>[18x]GAMGNQKTKASKLETAAKNLENQNKQEYIKINEIDAQGINFLATFKADEKDNLSQYEEMQIKRTIYSSLNYEKQKINTLKEILETLYNKLQHRYTSKEFIYQIVASIQYDIDRVLCLIKEAIIKDNLHTQNQKESELLMNLDSSLKTRQNFAKKLNETIDDYNKDSKNIQTNVDALATYMKENYKTLDSFKPIN

Two CspA orthologous proteins, BGA71 and BGA66, that are capable of binding complement system components C7, C8, and C9 and thus inhibiting the assembly of the MAC have been identified in B. bavariensis, allowing B. bavariensis to escape the attack by the immune system. The importance of BGA71 and BGA66 in the resistance to the immune system was supported by the gain of resistance to complement-mediated killing after expression of either protein in the serum-sensitive B. garinii strain G132. In conclusion, we have solved the crystal structure of the key complement inhibitory protein BGA71 from B. bavariensis. The overall fold of the BGA71 protein looks similar (Cα root-mean-square deviation from 1.66 Ǻ to 2.63 Ǻ) to the previously released crystal structures of the orthologous PFam54 proteins CspA, BBA64, BBA66, and BBA73 of B. burgdorferi.

All three BGA71 constructs were overexpressed in E. coli, but only BGA7162-251 yielded crystals, suggesting that the flexible region present in the other two constructs interfered with the crystal formation, as previously observed for the BBA66 protein of B. burgdorferi. The diffracting crystals of the Se-Met BGA7162-251 construct belonged to the space group P31 and contained 18 molecules per asymmetric unit with a water content of approximately 45%. The final model of BGA7162-251 was generated for residues 69–251 since the first four residues that remained after cleavage of the His-tag and residues 66–68 were not built due to weak electron density. By surveying the crystal structure of BGA71, we identified cysteine 173 in α-helix D as the residue that forms disulfide bridges, which is responsible for cross-linking of the two monomers. Furthermore, comparative sequence analysis of the PFam54 orthologous proteins reveals that cysteine 173 is not present in any other orthologous PFam54 protein, suggesting that dimerization by cysteine cross-linking is a unique feature of BGA71. The structure of CspA showed the highest similarity to BGA71 among the other PFam54 orthologs of B. burgdorferi, with a Cα root-mean-square deviation of 1.66 Ǻ. While BGA71 did not bind CFH and CFHL-1, an interaction with components C7 and C9 has been demonstrated. However, the lack of binding complement regulators can be explained by the inability of BGA71 to form a homodimer in the same manner as CspA. However, the proposed N-terminal residues 37–63 involved in the binding of C7 and C9 are not visible in the crystal structure of BGA71 since they form a flexible loop region connecting the protein structural domain to the cell surface.>MTDMNILDLFLKASLLVKLIMLILIGFSIASWAIIIQRTRILNAAAREAEAFEDKFWSGIELSRLYQESQGKRDNLTGSEQIFYSGFKEFVRLHRANSHAPEAVVEGASRAMRISMNRELENLETHIPFLGTVGSISPYIGLFGTVWGIMHAFIALGAVKQATLQMVAPGIAEALIATAIGLFAAIPAVMAYNRLNQRVNKLELNYDNFMEEFTAILHRQAFTVSESNKG[5x];>[2x]MARARGRGRRDLKSEINIVPLLDVLLVLLLIFMATAPIITQSVEVDLPDATESQAVSSNDNPPVIVEVSGIGQYTVVVEKDRLERLPPEQVVAEVSSRFKANPKTVFLIGGAKDVPYDEIIKALNLLHSAGVKSVGLMTQPI;> MSKATEQNDKLKRAIIISAVLHVILFAALIWSSFDENIEASAGGGGGSSIDAVMVDSGAVVEQYKRMQSQESSAKRSDEQRKMKEQQAAEELREKQAAEQERLKQLEKERLAAQEQKKQAEEAAKQAELKQKQAEEAAAKAAADAKAKAEADAKAAEEAAKKAAADAKKKAEAEAAKAAAEAQKKAEAAAAALKKKAEAAEAAAAEARKKAATEAAEKAKAEAEKKAAAEKAAADKKAAAEKAAADKKAAE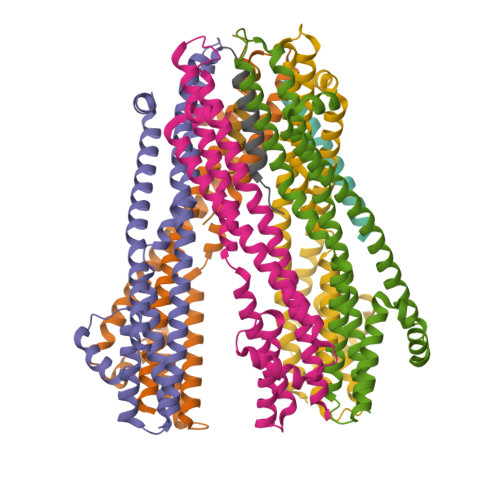KAAAEKAAADKKAAAEKAAADKKAAAAKAAAEKAAAAKAAAEADDIFGELSSGKNAPKTGGGAKGNNASPAGSGNTKNNGASGADINNYAGQIKSAIESKFYDASSYAGKTCTLRIKLAPDGMLLDIKPEGGDPALCQAALAAAKLAKIPKPPSQAVYEVFKNAPLDFKP> GAGCAGACGTGACG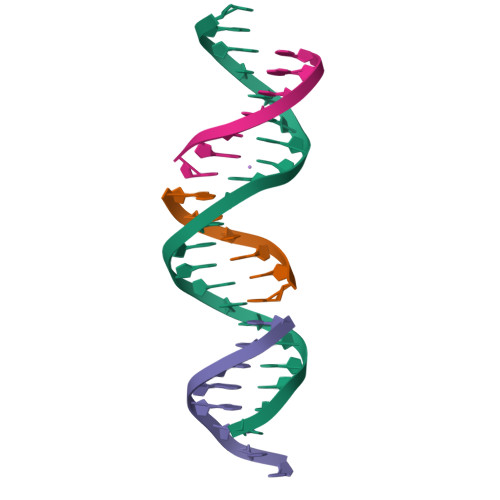AGACTCA;> TCGTCA;> TCTGAGTC;> CGTCTGC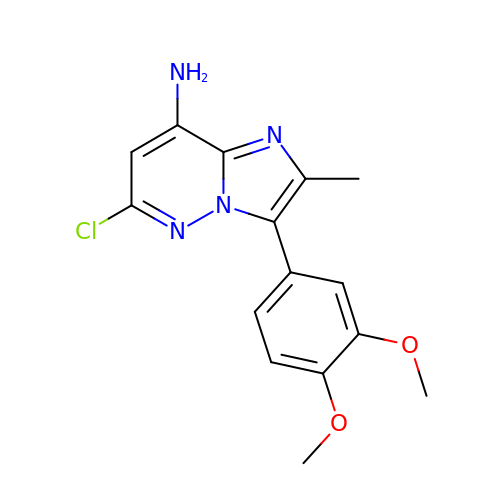6-chloro-3-(3,4-dimethoxyphenyl)-2-methylimidazo[1,2-b]pyridazin-8-amine | C15 H15 Cl N4 O2 | QKMGMIGTYUUELE-UHFFFAOYSA-N1-(2-ethyl-1,3-thiazol-5-yl)-N-methylmethanamine 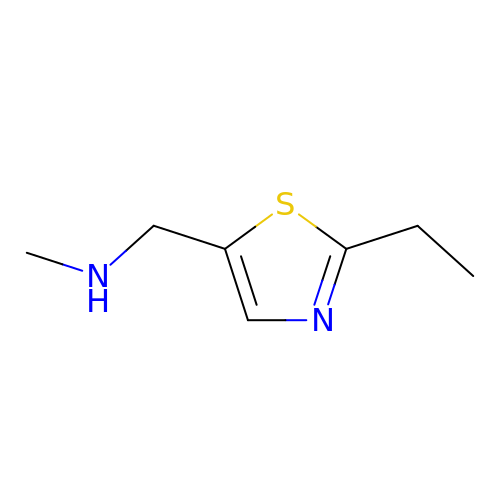| C7 H12 N2 S | CSZFIJNBBMUGDN-UHFFFAOYSA-N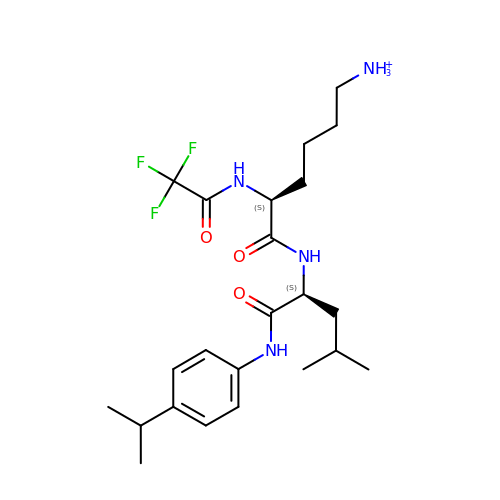6-ammonio-N-(trifluoroacetyl)-L-norleucyl-N-[4-(1-methylethyl)phenyl]-L-leucinamide | C23 H36 F3 N4 O3 | OSCPPTDAQZTYFO-OALUTQOASA-O>DRHHHHHHKLNLTCPACKVLFTALNHGLKKEPNVARVGSVAIKICKM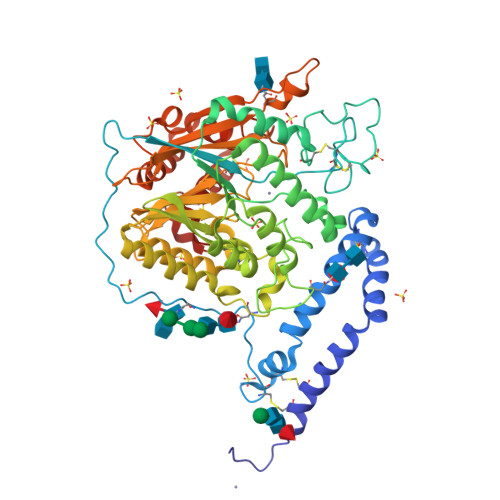LNIAPLDVCQSAVHLFEDDVVEVWTRSVLSPSEACGLLLGSSCGHWDIFSTWNISLPSVPKPPPKPPSPPAPGAPVSRVLFLTDLHWDHEYLEGTDPYCADPLCCRRGSGWPPNSQKGAGFWGEYSKCDLPLRTLESLLKGLGPAGPFEMVYWTGDIPAHDVWQQSRQDQLRALTTITDLVRKFLGPVPVYPAVGNHESTPVNGFPPPFIKGNQSSQWLYEAMAKAWEPWLPADALHTLRIGGFYALTPRPGLRLISLNMNFCSRENFWLLINSTDPAGQLQWLVEELQAAENRGDKVHIIGHIPPGHCLKSWSWNYYKIIARYENTLAGQFFGHTHVDEFEIFYDEETLSRPLAVAFLAPSATTFINLNPGYRVYQIDGNYPGSSHVVLDHETYILNLTQANAAGGTPSWKRLYRARETYGLPDAMPASWHNLVYRMRDDEQLFQTFWFLYHKGHPPSEPCGTPCRLATLCAQLSARADSPALCRHLMPN[2x]> MHHHHHHMPIIEQVRAREILDSRGNPTVEVEVALIDGTFARAAVPSGASTGEHEAVELRDGGDRYGGKGVQKAVQAVLDEIGPAVIGLNADDQRLVDQALVDLDGTPDKSRLGGNAILGVSLAVAKAAADSAELPLFRYVGGPNAHILPVPMMNILNGGAHADTAVDIQEFMVAPIGAPSFVEALRWGAEVYHALKSVLKKEGLSTGLGDEGGFAPDVAGTTAALDLISRAIESAGLRPGADVALALDAAATEFFTDGTGYVFEGTTRTADQMTEFYAGLLGAYPLVSIEDPLSEDDWDGWAALTASIGDRVQIVGDDIFVTNPERLEEGIERGVANALLVKVNQIGTLTETLDAVTLAHHGGYRTMISHRSGETEDTMIADLAVAIGSGQIKTGAPARSERVAKYNQLLRIEEALGDAARYAGDLAFPRFACET

Enolase, a ubiquitous enzyme, catalyzes the reversible conversion of 2-phospho­glycerate (2PG) to phospho­enolpyruvate (PEP) in the glycolytic pathway of organisms of all three domains of life. Here we present structural snapshots of Mycobacterium tuberculosis (Mtb) enolase in apo, PEP-bound and two 2PG-bound forms as it catalyzes the conversion of PEP to 2PG. MtEno has a topology similar to other enolase structures, a smaller N-terminal domain and a larger C-terminal domain. The crystal and the cryoEM structures (enzyme in solution, frozen) along with the biochemical studies clearly demonstrate that the functional unit of MtEno is an octamer.

The octameric fraction was further used for structural studies. The structure of enolase in the apo state was determined using both cryoEM and X-ray crystallography. One of them, described here as IF1, is similar to the interface observed in conventional dimers, whereas the other, IF2, exists in between two neighboring dimers and has only been reported in bacterial enolases. Further, the MtEno crystal structure was superposed with its Synechococcus elongates counterpart with which it showed a low RMSD of 0.65 Å. The protein overall fold is highly conserved, except for a small conformational variation in loop 1 [Fig. S4(a)]. Notably, the pK a of Lys335 is estimated to be ∼11.5 in the MtEno WT apo state, unable to facilitate a reduction reaction on the carbanion intermediate.>MAHHHHHHVGTNDANIADVVTKVLGEYGAPGAVSVAALTAKSPDGKSNSSADADVVARMVAKAIRDHAGTAQPSGNAATSSAAVSDGV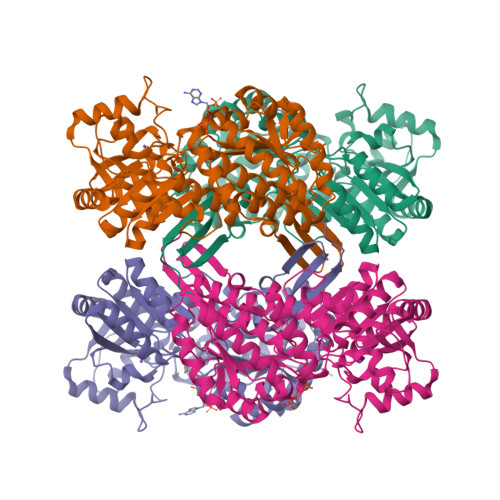FETMDAAVEAAALAQQQYLLCSMSDRARFVQGIRDVILNQDTLEKMSRMAVEETGMGNYEHKLIKNRLAGEKTPGIEDLTTDAFSGDNGLTLVEYSPFGVIGAITPTTNPTETIVCNSIGMLAAGNSVVFSPHGRARQVSLLLVRLINQKLAALGAPENLVVTVEKPSRENTLAMMAHPKVRMLVATGGPALVKAVLSTGKKAIGAGAGNPPVVVDETANIEKAACDIVNGCSFDNNITCTAEKEIIAVAQIADYLIFNLKKNGAYEIKDPAVLQQLQDLVLTAKGGPQTKCVGKSAVWLLSQIGISVDASIKIILMEVPREHPFVQEELMMPILPLVRVETVDDAIDLAIEVEHDNRHTAIMHSTDVRKLTKMAKLIQTTIFVKNGPSYAGHGAGGEGYSTFTIAGPTGEGLTSAKSFARRRKCVMVEALNIR[10x]> MRGSHHHHHHTDPQGDAAQKTDTSHHDQDHPTFNKITPNLAEFAFSLYRQLAHQSNSTNIFFSPVSIATAFAMLSLGTKADTHDEILEGLNFNLTEIPEAQIHEGFQELLRTLNQPDSQLQLTTGNGLFLSEGLKLVDKFLEDVKKLYHSEAFTVNFGDTEEAKKQINDYVEKGTQGKIVDLVKELDRDTVFALVNYIFFKGKWERPFEVKDTEEEDFHVD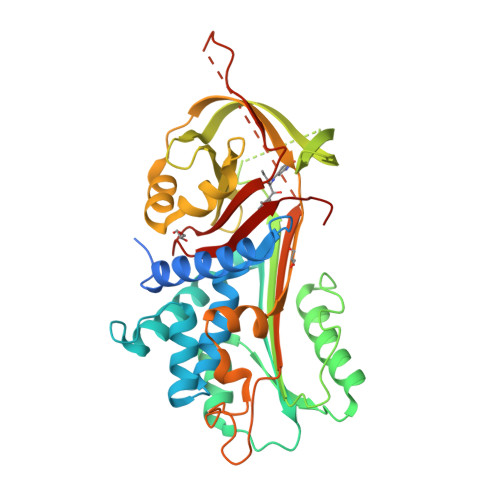QVTTVKVPMMKRLGMFNIQHSKKLSSWVLLMKYLGNATAIFFLPDEGKLQHLENELTHDIITKFLENEDRRSASLHLPKLSITGTYDLKSVLGQLGITKVFSNGADLSGVTEEAPLKLSKAVHKAVLTIDEKGTEAAGAMFLEAIPMSIPPEVKFNKPFVFLMIEQNTKSPLFMGKVVNPTQ> MTQLRVAFSAARTANFAPGTLDQPIAFDLLHTNLGDMFDTGSGRFTCPATGAYVFIFHILKLAISVPLYINLMRNEEVMVSAYANDGAPDHETASNHA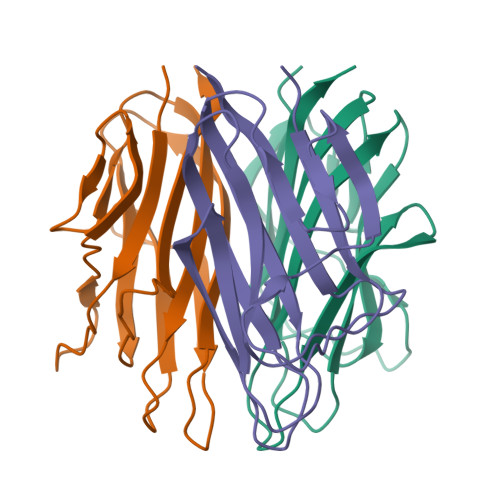VLQLFQGDQVWLRLHRGAIYGSSWKYSTFSGFLLYQDLEHHHHHH The Linker of Nucleoskeleton and Cytoskeleton (LINC) complex crosses both inner and outer nuclear membranes of the nuclear envelope to mechanically transduce cytoskeletal forces to nuclear contents. It is formed of nuclear SUN (Sad1 and UNC84 homology) and cytoplasmic KASH (Klarsicht, ANC-1, and Syne homology) proteins, which interact within the nuclear lumen. JAW1/LRMP (lymphoid restricted membrane protein) is an atypical KASH protein that is localised in the endoplasmic reticulum and outer nuclear membrane, and is specifically expressed in certain cells of the immune system, small intestine, pancreas and taste buds. Here, we report the crystal structure of the SUN-KASH complex between SUN1 and the non-canonical KASH domain of JAW1/LRMP (herein referred to as KASH6).

Thus, we crystallised the SUN1-KASH6 complex and solved its X-ray crystal structures from several crystals at resolutions between 1.7 and 2.3 Å. In contrast with previous SUN-KASH 6:6 structures, the SUN1-KASH6 crystal structure contains nine SUN domains, such that head-to-head interfaces of three SUN1 trimers interact together around a three-fold symmetry axis in a ‘trimer-of-trimers’ configuration. KASH6 peptides are clearly bound at both of these KASH-binding pockets of each SUN1 trimer (these are herein referred to as KASH6α and KASH6β). The third KASH-binding pocket of each SUN1 trimer is located on the underside of the trimer-of-trimers structure, away from inter-trimer interfaces. In other crystal structures, at resolutions of 2.0 Å and 2.3 Å, we observed no third peptide, with the KASH-binding pocket containing only water molecules. In absence of KASH6γ, the remaining structure was essentially unaltered (r.m.s. deviation = 0.1 Å). Hence, the third binding pocket on the lower surface of the trimer-of-trimers structure cannot stably bind to a KASH6 peptide. We conclude that the SUN1-KASH6 structure is a 9:6 complex in which three SUN1 trimers are bound to six KASH6 peptides. Further, their distinct conformations mean that all KASH6α and KASH6β peptides of the structure are oriented with their N-termini directed towards the top surface of the molecule. This asymmetry within the SUN1-KASH6 trimer-of-trimers structure positions all six stably bound KASH6 peptides in a manner that is suitable for the insertion of their immediately upstream transmembrane helices into the outer nuclear membrane.

>[3x]GSGGSGGITEAQARAIVNSALKLYSQDKTGMVDFALESGGGSILSTRCSETYETKTALMSLFGIPLWYFSQSPRVVIQPDIYPGNCWAFKGSQGYLVVRLSMMIHPAAFTLEHIPKTLSPTGNISSAPKDFAVYGLENEYQEEGQLLGQFTYDQDGESLQMFQALKRPDDTAFQIVELRIFSNWGHPEYTCLYRFRVHGEPVK;>GSMTGQLFQKSVDAAPTQQEDSWTSLEHILWPFTRLRHNGPPPV[2x]> MAGQTTVDSRRQPPEEVDVLVVGAGFSGLYALYRLRELGRSVHVIETAGDVGGVWYWNRYPGARDDIESIEYCYSFSEEVLQEWNWTERYASQPEILRYINFVADKFDLRSGITFHTTVTAAAFDEATNTWTVDTNHGDRIRARYLIMASGQLSVPQLPNFPGLKDFAGNLYHTGNWPHEPVDFSGQRVGVIGTGSSGIQVSPQIAKQAAELFVFQRTPHFAVPARNAPLDPEFLADLKKRYAEFREESRNTPGGTHRYQGPKSALEVSDEELVETLERYWQEGGPDILAAYRDILRDRDANERVAEFIRNKIRNTVRDPEVAERLVPKGYPFGTKRLILEIDYYEMFNRDNVHLVDTLSAPIETIT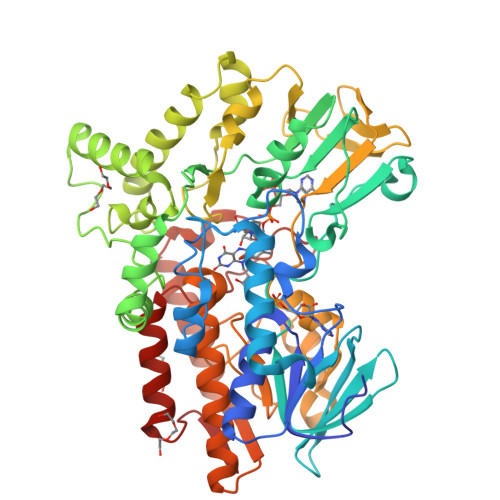PRGVRTSEREYELDSLVLATGFDALTGALFKIDIRGVGNVALKEKWAAGPRTYLGLSTAGFPNLFFIAGPGSPSALSNMLVSIEQHVEWVTDHIAYMFKNGLTRSEAVLEKEDEWVEHVNEIADETLYPMTASWYTGANVPGKPRVFMLYVGGFHRYRQICDEVAAKGYEGFVLT> SDFTLNGIKVEDTFAEAFDVAGTAIIVTNDTPKWAMIAATVMTGFATSVIGCGAEAGIDAELSPDETPDGRPGVRILLFGFEPNGLKDQLLKRVGQCILTCPGTACFAGVEGPTKIKLGGAIRYFGDGFAVAKRLPDHEGKMR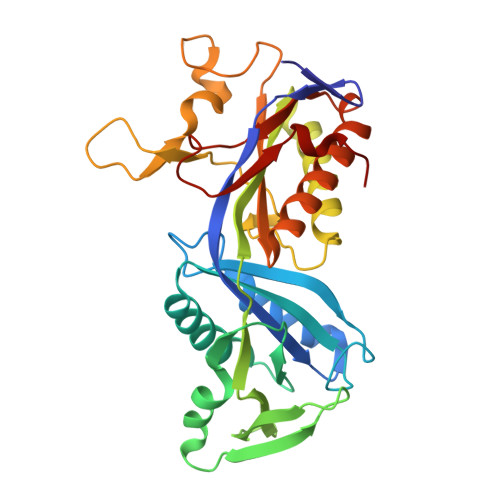RYWRIPVMDGEFLCEDSVRAVDGAVGGGNLLFLGRKHADTLIVAEIAVEAAKAIPGAILPFPGGIVRSGSKVGGRTKGMMASTNDAYCPTLKGRAGSALPPECGVVLEIVIDALTSAAVAESMRAALHAATEIGAQHGLVAVTAGNYGGNLGRHHYHLRDLLEKPAA> AKPKIDKDFKGKANPDTPRVDKDTPVNHQVGDVVEYEIVTKIPALANYATANWSDRMTEGLAFNKGTVKVTVDDVALEAGDYALTEVATGFDLKLTDAGLAKVNDQNAEKTVKITYSATLNDKAIVEVPESNDVTFNYGNNPDHGNTPKPNKPNENGDLTLTKTWVDATGAPIPAGAEATFDLVNAQAGKV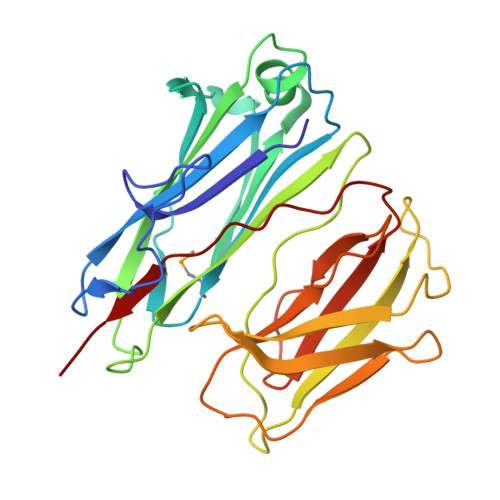VQTVTLTTDKNTVTVNGLDKNTEYKFVERSIKGYSADYQEITTAGEIAVKNWKDENPKPLDPTEPKVVTYG>[8x]MALVDGFLELERSSG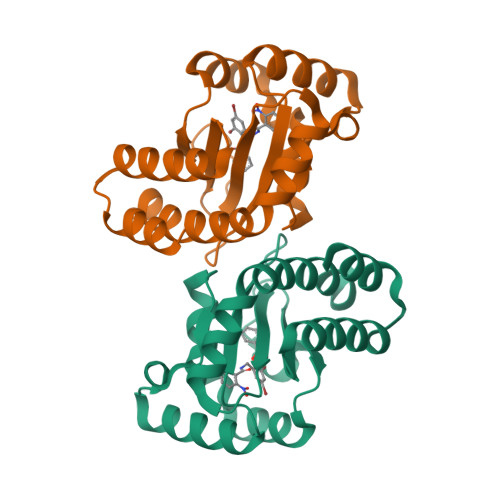KLEWSAILQKMASDLGFSKILFGLLPKDSQDYENAFIVGNYPAAWREHYDRAGYARVDPTVSHCTQSVLPIFWEPSIYQTRKQHEFFEEASAAGLVYGLTMPLHGARGELGALSLSVEAENRAEANRFMESVLPTLWMLKDYALQSGAGLAFEHP>GAFLIRTWVTLKAEQTILPLVDEALQHTTTKGIVFQHPEIVAHMDLMREDLHLEPFYWKLPEQFEGKKLMAYGGKLKYAIYFEAREETGFSTYNPQVIIRGGTPTHARIIVRHMAAPLIGQLTRHEIEMTEKEWKYYGDDPRVHRTVTREDFLDI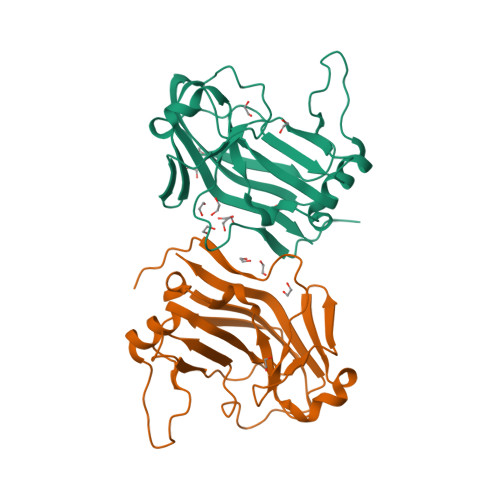LYDIHYILIKATYGNFMRQSRISEISMEVA[2x]>[3x]LLIFIYLLLMAVAVFLVYQTIMDFREKLKHPVMSVSYKEVDRYDAPGIALYPGQAQLLSCKHYYEVIPPLRSPGQPGDV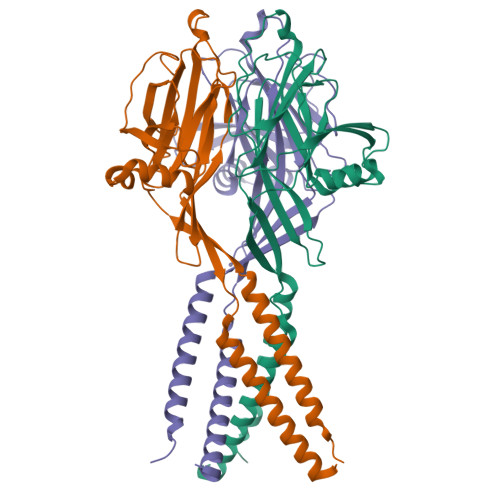NCTTQRVNYTDPFSNQTLKSALIVRGPREVQKRELVFLQFRLNQSSEDFSAIDYLLFSSFQEFLQSPDRAGFMQACESAYSSWKFSGGFRTWVKMSLVETKEEDGREAVEFRQETSVVNYIDQRPAAEKSAQLFFVVFEWKDPFIQKVQDIITANPWNTIALLCGAFLALFKAAEFAKLSVKWMA>MVTVGNYCEAEGPVGPAWMQDGLSPCFFFTLVPSTRMALGTLALVLALPCRRRERPAGADSLSWGAGPRISPYVLQLLLATLQAALPLAGLAGRVGTARGAPLPSYLLLASVLESLAGACGLWLLVVERSQARQRLAMGIWIKFRHSPGLLLLWTVAFAAENLALVSWNSPQWWWARADLGQQVQFSLWVLRYVVSGGLFVLGLWAPGLRPQSYTLQVHEEDQDVERSQVRSAAQQSTWRDFGRKLRLLSGYLWPRGSPALQLVVLICLGLMGLERALNVLVPIFYRNIVNLLTEKAPWNSLAWTVTSYVFLKFLQGGGTGSTGFVSNLRTFLWIRVQQFTSRRVELLIFSHLHELSLRWHLGRRTGEVLRIADRGTSSVTGLLSYLVFNVIPTLADIIIGIIYFSMFFNAWFGLIVFLCMSLYLTLTIVVTEWRTKFRRAMNTQENATRARAVDSLLNFETVKYYNAESYEVERYREAIIKYQGLEWKSSASLVLLNQTQNLVIGLGLLAGSLLCAYFVTEQKLQVGDYVLFGTYIIQLYMPLNWFGTYYRMIQTNFIDMENMFDLLKEETEVKDLPGAGPLRFQKGRIEFENVHFSYADGRETLQDVSFTVMPGQTLALVGPSGAGKSTILRLLFRFYDISSGCIRIDGQDISQVTQASLRSHIGVVPQDTVLFNDTIADNIRYGRVTAGNDEVEAAAQAAGIHDAIM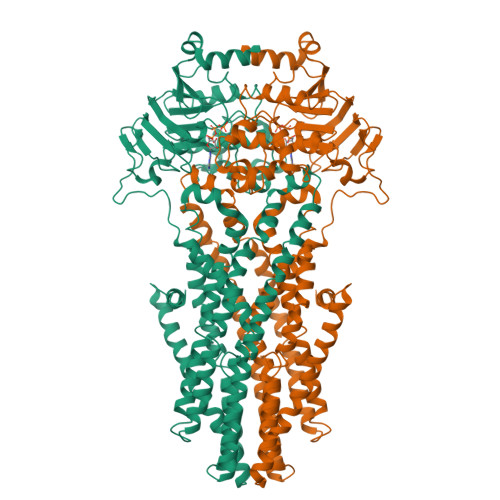AFPEGYRTQVGERGLKLSGGEKQRVAIARTILKAPGIILLDQATSALDTSNERAIQASLAKVCANRTTIVVAHRLSTVVNADQILVIKDGCIVERGRHEALLSRGGVYADMWQLQQGQEETSEDTKPQTMER[2x]> YFQGMQLRFARLSEHATAPTRGSARAAGYDLYSAYDYTIPPMEKA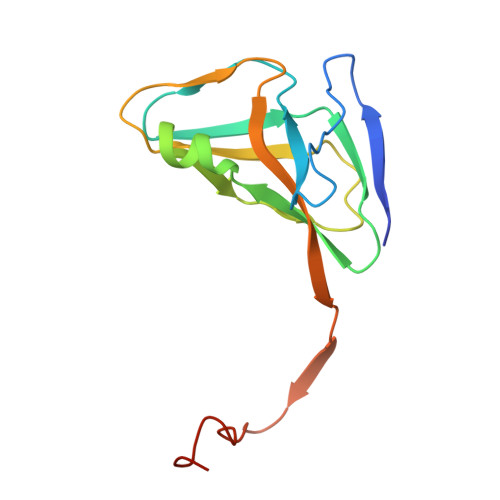VVKTDIQIALPSGCYGRVAPRSGLAAKHFIDVGAGVIDEDYRGNVGVVLFNFGKEKFEVKKGDRIAQLICERIFYPEIEEVQALDDTERGSGGFGSTGKN>HMCDSALTAQANDLRIYQVMVESFVNGDDAIGHGTGYGTSHHKGDLQGIIDSLDYIESLGMNAIWLTPIFDSIPVEGQDHWADRLDATGYFTSNYFAVDPRFGTMEQAKELVEKAHEKGLYVFFDGVFGHHKDNVVPSPEGRLPVGENNPVSYPESLAFYQEVATFWIEELKIDGWRLDQAYQVPTEAWTAIRASVDEASKSVTYVNSKGEAVNPLGYMVAEIWNNENYIKETGYGAEGEPALCSAFDFPVRYRVVETFAANENGIGNKGGKWLDEGMNLHRLYPSHAQPNLMLGNHDLVRFGDLLQRGNIASPEQAEYWERHKAALSFQAAYSGPITLYYGEEIGDELEGYAQKVEQDCAVQGLCDDHVARTSANIDGLTVNLNEKQRDLKQYVSQLMTLRAAHPALSRGERTNIVANETVYIDHKQADDDALIYMVSTTADQDTVELKASDIASDGQLVDLLTGKVHSAINGEYQISLAPFEAKFLLIETPSASGLTKVATVSAASSLIGEGFMAQCDNPTIEGDGPIGKTL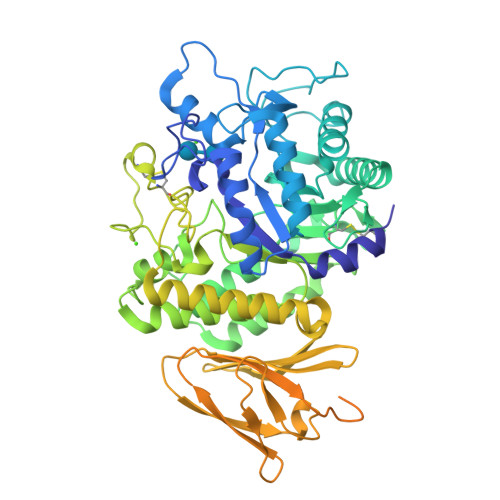YVVGDFADASWKQKPHRAYRYVGENTYQAVVDEKAGAFRMQYASKDWSPQFTADGLELTPGKTASLKRGGYGQDTAVTLPEAGQYVWSLKFTDSGDPEQIMVSKCP[4x]>MERAFIEWYPRGYGVAFKIKKKIYEKLSKYQKIEVYETEGFGRLLALDGTVQLVTLGERSYHEPLVHPAMLAHPKPKRVLVIGGGDGGTVREVLQHDVDEVIMVEIDEDVIMVSKDLIKIDNGLLEAMLNGKHEKAKLTIGDGFEFIKNNRGFDVIIADSTDPVGPAKV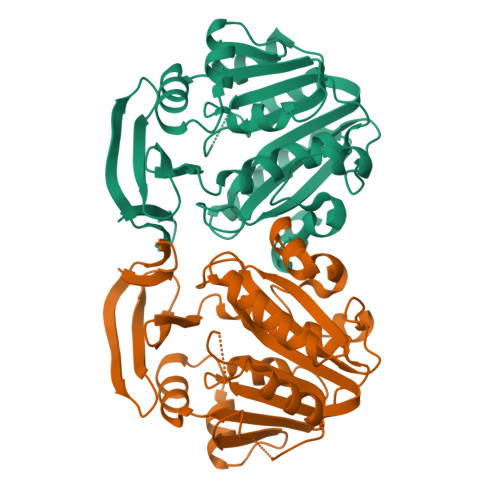LFSEEFYRYVYDALNNPGIYVTQAGSVYLFTDELISAYKEMKKVFDRVYYYSFPVIGYASPWAFLVGVKGDIDFTKIDRERAKKLQLEYYDPLMHETLFQMPKYIRETLQRL[2x]(5S,11R)-5,8,11-trihydroxy-5,11-dioxido-17-oxo-4,6,10,12,16-pentaoxa-5,11-diphosphaoctadec-1-yl pentadecanoate | C26 H52 O13 P2 | 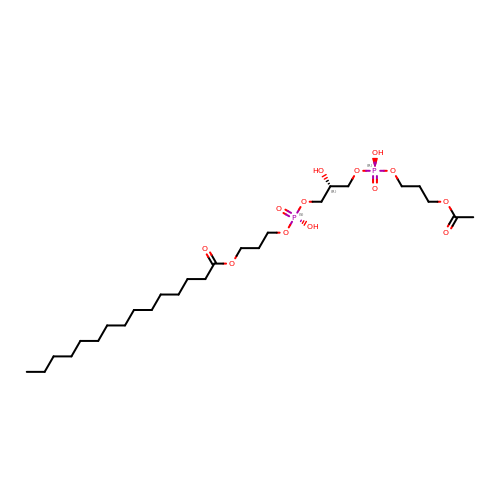UKWPDXFRXMWSMQ-VWLOTQADSA-N> ERAGPVTWVMMIACVVVFIAMQILGDQEVMLW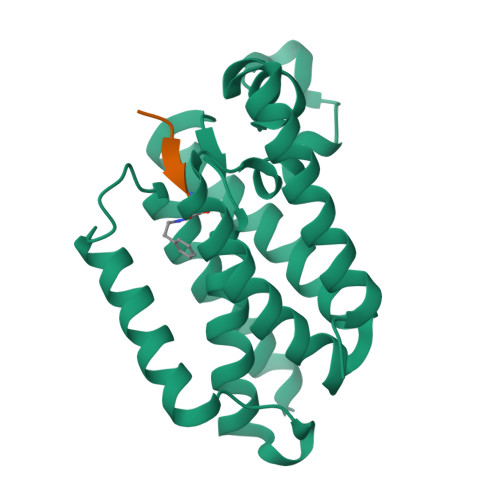LAWPFDPTLKFEFWRYFTHALMHFSLMHILFNLLWWWYLGGAVEKRLGSGKLIVITLISALLSGYVQQKFSGPWFGGLSGVVYALMGYVWLRGERDPQSGIYLQRGLIIFALIWIVAGWFDLFGMSMANGAHIAGLAVGLAMAFVDSL>[2x]MAGSYNYAEALQKAIYFYECQQAGPLPEWNRVEWRGDATMNDEVLGGWYDAGAHVKFNLPMAYSAAMLGWALYEYGDDIEASGQRLHLERNLAFALDYLVACDRGDSVVYQIGDGAADHKWWGSAEVIEKEMTRP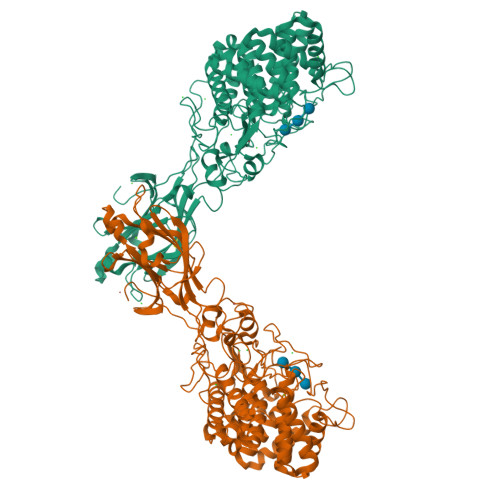YFVGKGSAVVGQMAAALAVGSIVLKNDTYLRYAKKYFELADATRSDSTYTAANGFYSSHSGFWDELLWASTWLYLATGDRNYLDKAESYTPKLNRQNQTTDIEYQWAHCWDDCHYGAMILLARATGKEEYHKFAQMHLDWWTPQGYNGKRVAYTPGGLAHLDTWGPLRYATTEAFLAFVYADSINDPALKQKYYNFAKSQIDYALGSNPDNRSYVVGFGNNPPQRPHHRTAHGTWLDKRDIPEKHRHVLYGALVGGPGRDDSYEDNIEDYVKNEVACDYNAGFVGALCRLTAEYGGTPLANFPPPEQRDDEFFVEAAINQASDHFTEIKALLNNRSSWPARLIKDLSYNYYMDLTEVFEAGYSVDDIKVTIGYCESGMDVEISPITHLYDNIYYIKISYIDGTNICPIGQEQYAAELQFRIAAPQGTKFWDPTNDFSYQGLTRELAKTKYMPVFDGATKIFGEVPGGLEHHHHHH Herein, we describe the use of GE to optimize a fragment‐derived inhibitor of Mycobacterium tuberculosis pantothenate synthetase, an attractive target for developing new drugs against tuberculosis. Pantothenate synthetase catalyzes the ATP‐dependent formation of an amide bond between pantoate and β‐alanine. The work presented here demonstrates the use of GE analysis to critically and thoroughly examine the binding distribution of a lead compound and illustrates the practicality of applying GE analysis to modify parts of a molecule that are not making efficient contributions to binding. In this case, it led to the generation of a relatively potent and bactericidal inhibitor of M. tuberculosis pantothenate synthetase.

Based on these observations, the initial optimization strategy was focused on replacement of the methyl pyridine and the benzofuran groups rather than the acyl sulfonamide linker in both compounds 5 and 8. Compounds were designed with the objective of optimizing interactions at the P1 or P2 sites of panthothenate synthetase. Consequently, 1‐ethyl‐3‐(3‐dimethylaminopropyl)‐carbodiimide (EDCI)‐mediated coupling reactions were employed to generate a series of indole acyl sulfonamide compounds (10–19; the syntheses are described in the Supporting Information). Compound 10 was the most ligand efficient compound tested. The GE value for the toluene group in 10 is 0.35—a marked improvement over the GE values of 0.17 and 0.16 for the methyl pyridine and benzofuran groups in 5 and 8, respectively. In order to establish this, the structures of the four most potent inhibitors (10–13) bound to the enzyme were solved using protein X‐ray crystallography. The X‐ray crystal structures of 10–13 bound to pantothenate synthetase show binding at the active site, with a conserved binding mode for the indole sulfonamide fragment core. Less obviously, the substituted groups on all four compounds were seen to bind in the P1 pocket of the enzyme. The P1 pocket binds the alkyl groups of the pantoate substrate and is primarily lipophilic, surrounded by the hydrophobic residues Pro 38, Met 40, Val 143, Leu 146 and Phe 157. In contrast, the P2 site binds the phosphates of ATP and is relatively hydrophilic. As can be seen in Figure 2, the binding orientations of the added groups are all similar, and no new hydrogen bonds are formed.

>[2x]MAIPAFHPGELNVYSAPGDVADVSRALRLTGRRVMLVPTMGALHEGHLALVRAAKRVPGSVVVVSIFVNPMQFGAGGDLDAYPRTPDDDLAQLRAEGVEIAFTPTTAAMYPDGLRTTVQPGPLAAELEGGPRPTHFAGVLTVVLKLLQIVRPDRVFFGEKDYQQLVLIRQLVADFNLDVAVVGVPTVREADGLAMSSRNRYLDPAQRAAAVALSAALTAAAHAATAGAQAALDAARAVLDAAPGVAVDYLELRDIGLGPMPLNGSGRLLVAARLGTTRLLDNIAIEIGTFAGTDRPDGYRAILESHWRN>VSVGTHPTFENSPSGTVLTSPPDGSAVDRATDAARRVVDALLRTDRGNANLERVAEELNSIAGHLEEHAPAVAERLIDMWNGEGVTRHDPVTGPENALAPPVVLEGLSDGSVRGTVTLTIPYQGPP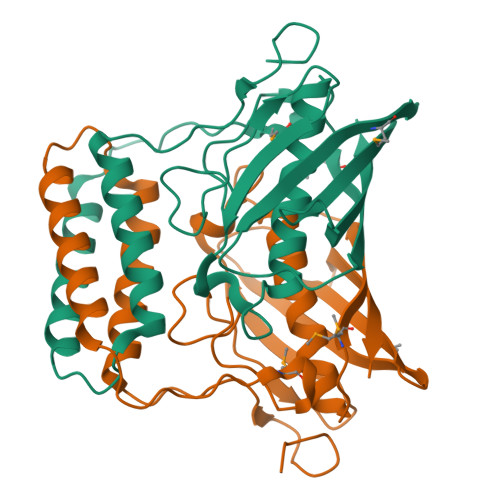GHVHGGVSALLLDHVLGVANAWGGKAGMTAQLSTRYHRPTPLFEPLTLTGKLMSVDGRKITTAGDIRTADGQVCVSVEGLFVDKTVPRPR[4x]> MRDADADAGGGADGGDGRGGHSCRGGVDTAAAPAGGAPPAHAPGPGRDAASAARGSRMRPHIFTLSVPFPTPLEAEIAHGSL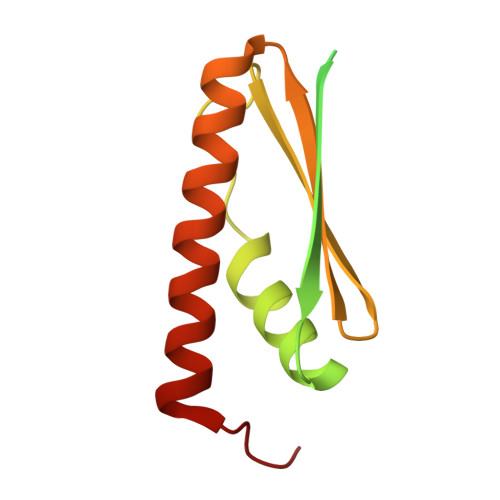APDAEPHQRVVGKDLTVSGRILVVRWKAEDCRLLRISVINFLDQLSLVVRTMQRFGPPVSR> AATTGYDAVDDLLHYHERGNGIQINGKDSFSNEQAGLFITRENQTWNGYKVFGQPVKLTFSFPDYKFSSTNVAGDTGLSKFSAEQQQQAKLSLQSWADVANITFTEVAAGQKANITFGNYSQDRPGHYDYGTQAYAFLPNTIWQGQDLGGQTWYNVNQSNVKHPATEDYGRQTFTHEIGHALGLSHPGDYNAGEGNPTYNDVTYAEDTRQFSLMSYWSETNTGGDNGGHYAAAPLLDDIAAIQHLYGANLSTRTGDTVYGFNSNTGRDFLSTTSNSQKVIFAAWDAGGNDTFDFSGYTANQRINLNEKSFSDVGGLKGNVSIAAGVTIENAIGGSGNDVIVGNAANNVLKGGAGNDVLFGGGGADEL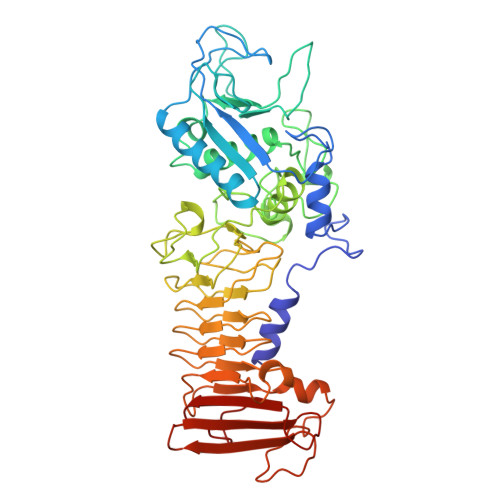WGGAGKDIFVFSAASDSAPGASDWIRDFQKGIDKIDLSFFNKEANSSDFIHFVDHFSGTAGEALLSYNASSNVTDLSVNIGGHQAPDFLVKIVGQVDVATDFIV> MSMLVVVTENVPPRLRGRLAIWLLEVRAGVYVGDVSAKIREMIWEQIAGLAEEGNVVMAWA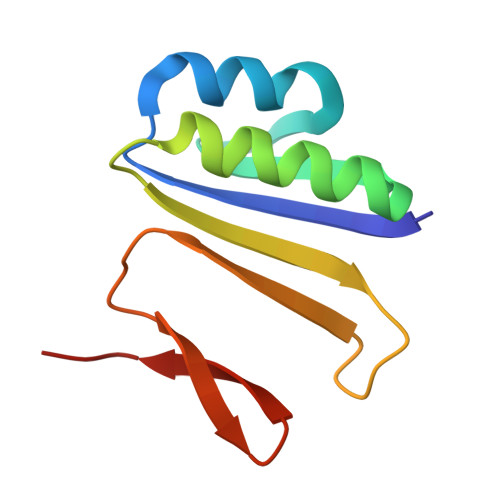TNTETGFEFQTFGLNRRTPVDLDGLRLVSFLPV>GPGLKQKIVIKVAMEGNNCRSKAMALVASTGGVDSVALVGDLRDKIEVVGYGIDPIKLISALRKKVGDAELLQVS[2x];> METGNKYIEKRAIDLSRERDPNFFDHPGIPVPECFWFMFKNNVRQDAGTCYSSWKMDMKVGPNWVHIKSDDNCNLSGDFPPGWIVLGKKRPGF

NLRs are a conserved component of plants' innate immune systems and survey the host environment for perturbations caused by invading pathogens. Intriguingly, the NLR pair Pik-1/Pik-2, which recognises AVR-Pik, also binds the effector via an HMA domain but this domain is integrated between the CC and NB-ARC regions of Pik-1. The integrated HMA domains of RGA5 and Pik-1 appear to have evolved from a family of rice proteins that only contain the HMA domain. Each of the Pikp-HMA monomers adopts the HMA-domain fold (Pfam: PF00403), comprising a four-stranded antiparallel β-sheet and two α-helices packed in an α/β sandwich.

However, following a co-expression strategy with 6xHis tagged Pikp-HMA and untagged AVR-PikD (see ‘Materials and methods’), we obtained crystals of this complex in multiple conditions. Optimisation of one of these conditions produced crystals diffracting X-rays to 1.6 Å resolution. The structure of the Pikp-HMA/AVR-PikD complex reveals an intimate interface formed between these proteins that buries 18.7% of the effector's solvent accessible surface area (1031.0 Å2). The majority of the interaction is formed with a monomer of Pikp-HMA, with 87.5% of the effector's buried surface area (902.2 Å2) and nine residues contributing hydrogen bond and/or salt bridge interactions. This suggests that the AVR-PikD/Pikp-HMA monomer interaction most likely represents the biologically significant interface. AVR-PikD adopts a six-stranded β-sandwich structure, stabilised by a di-sulphide bond between Cys54 and Cys70. Three primary sites of interaction are apparent between Pikp-HMA and AVR-PikD. The first is dominated by main-chain hydrogen bonding between the C-terminal β-stand of Pikp-HMA and β3 of AVR-PikD, which results in formation of a continuous antiparallel β-sheet comprising the four β-strands of Pikp-HMA and β3–5 of AVR-PikD. The second involves the side chain of Pikp-HMAAsp224, which forms a salt–bridge interaction with the side chain of AVR-PikDArg64, and is also held in place by a hydrogen bond of its main chain NH group to the side chain of AVR-PikDAsp66. AVR-PikDHis46 is bound in a pocket on Pikp-HMA via hydrogen bonds/salt bridge interactions between AVR-PikDHis46:Nδ1/Pikp-HMASer218:Oγ and AVR-PikDHis46:Nε2/Pikp-HMAGlu230:Oε1; also, Pikp-HMAVal232 packs on top of the AVR-PikDHis46 ring and contributes hydrophobic/van der Waals interactions.>[2x]MLSFLLTLKRMLRACLRAWKDKEFQVLFVLTILTLISG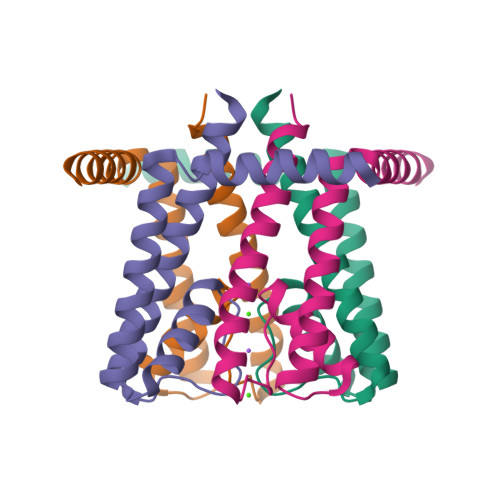TIFYSTVEGLRPIDALYFSVVTLTTVGEGNFSPQTDFGKIFTILYIFIGIGLVFGFIHKLAVNVQLPSILSNLVPR> GACATCACAGTGGACTACAAG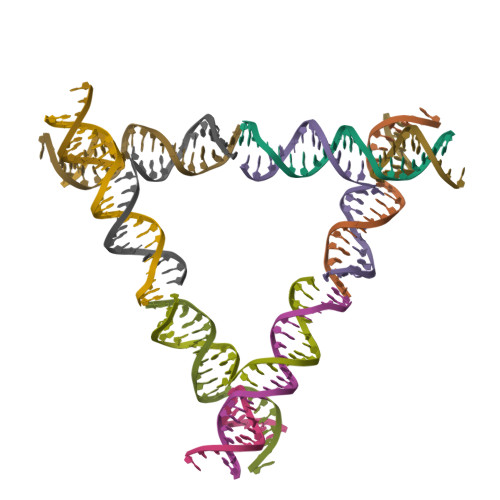;> TCCTTGTAGTGGAGTGT;> GAACACTCCTGAGACTACAA;> CTTGTAGTCTCACCACTGTGATGT>XSLSDKDKAAVKLLWSKISKSSDAIGNDALSRMIVVYPQTKTYFAHWPDLSPGSPHVKAHGKTVMGGIALAVSKIDDLRAGLLDLSEQHAYKLRVDPANFKILSHCILVVISMMFPKEFTPEAHVSLDKFLSGVSLALSERYR[2x];>VEWTDQERATISSIFGSLDYDDIGPKALSRCLIVYPWTQRHFGSFGNLYNAEAIIGNQKVAAHGIKVLHGLDRAVKNMDNIKEIYAELSILHSEKLHVDPDNFKLLADCLTIVVAAKMGSGFNPGTQATFQKFL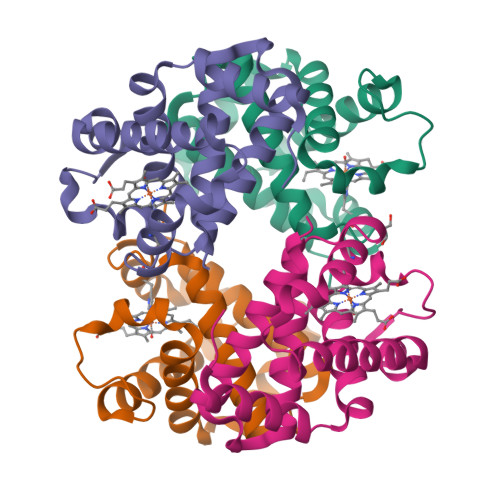AVVVSALGKQYH[2x]>[14x]TTTVGITLKDAVIMATERRVTMENFIMHKNGKKLFQIDTYTGMTIAGLVGDAQVLVRYMKAELELYRLQRRVNMPIEAVATLLSNMLNQVKYMPYMVQLLVGGIDTAPHVFSIDAAGGSVEDIYASTGSGSPFVYGVLESQYSEKMTVDEGVDLVIRAISAAKQRDSASGGMIDVAVITRKDGYVQLPTDQIESRIRKLGLIL;>AYDRAITVFSPDGRLFQVEYAREAVKKGSTALGMKFANGVLLISDKKVRSRLIEQNSIEKIQLIDDYVAAVTSGLVADARVLVDFARISAQQEKVTYGSLVNIENLVKRVADQMQQYTQYGGVRPYGVSLIFAGIDQIGPRLFDCDPAGTINEYKATAIGSGKDAVVSFLEREYKENLPEKEAVTLGIKALKSSLEEGEELKAPEIASITVGNKYRIYDQEEVKKFL[7x];>KRAALIQNLRDSYTETSSFAVIEEWAAGTLQEIEGIAKAAAEAHGVIRNSTYGRAQAEKSPEQLLGVLQRYQDLCHNVYCQAETIRTVIAIRIPEHKEEDNLGVAVQHAVLKIIDELEIKTLGSGEKSGSGGAPTPIGMYALREYLSARSTVEDKLLGSVDAESGKTKGGSQSPSLLLELRQIDADFMLKVELATTHLSTMVRAVINAYLLNWKKLIQPRTGTDHMFS[7x];>RAITVFSPDGRLFQVEYAREAVKKGSTALGMKFANGVLLISDKKVRSRLIEQNSIEAIQLIDDYVAAVTSGLVADARVLVDFARISAQQEKVTYGSLVNIENLVKRVADQMQQYTQYGGVRPYGVSLIFAGIDQIGPRLFDCDPAGTINEYKATAIGSGKDAVVSFLEREYKENLPEKEAVTLGIKALKSSLEEGEELKAPEIASITVGNKYRIYDQEEVKKFL[7x]

In archaea, the 20S is composed of homo-heptameric α- and β-rings, and PAN (Proteasomal Activator Nucleotidase), a homohexamer proteasomal ATPase, is the RP found in many species. Unfolded substrates enter the chamber through a narrow pore in the center of α-rings, where N-termini of α-subunits form a gate to impede unregulated access to the proteolytic chamber. We designed and assembled in vitro various asymmetric archaea 20S, in which one of the two α-rings contains a point mutation, K66A, which prevents RP binding to the α-ring. Our studies reveal that, upon binding of a RP with a conserved C-terminal HbYX motif to one α-ring, the gate of the opposite α-ring opens allosterically, resulting in similar proteolytic activities of 20S singly capped and doubly capped with PAN.

PA26 is a heptameric 11S activator from Trypanosoma brucei. To test whether the HbYX motif is a required element for inducing allosteric communication between the two distant α-rings, we further determined the structure of the asymmetric CP αWTββαK66A in complex with a single PA26, which does not have an HbYX motif grafted to its C-terminus. As expected, the gate in the proximal α-ring is open and there is no rotation of the α-subunit, but the activation loop of PA26 is engaged with the reverse turn loop of CP. In contrast to the results using PAN and PA26PANc, in an asymmetric proteasome bearing PA26, the gate of the distal α-ring is closed. This result suggests that binding a proteasomal activator without a C-terminal HbYX motif to one α-ring opens the proximal gate only, but does not induce allosteric opening of the distal gate. Indeed, the peptidase activity of symmetric CP doubly capped by PA26 is about twice that of the singly capped asymmetric CP, as predicted from the structures and the stated hypothesis. However, when bound with PA26, which does not have a C-terminal HbYX motif, peptidase activity of doubly capped proteasomes is greater than for those with a single cap.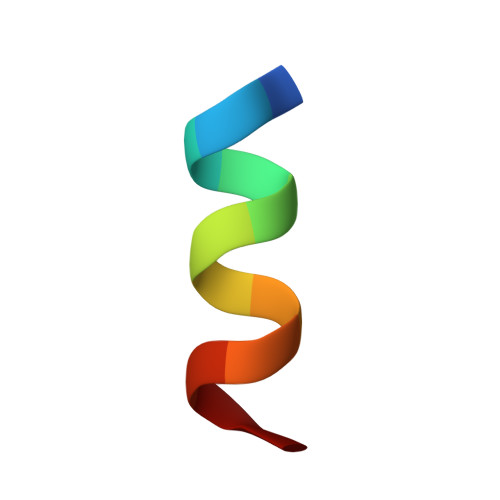> WEEWDREIENYT(2~{R},3~{S},4~{R},5~{R},6~{S})-2-(hydroxymethyl)-6-[5-(4-methylphenyl)-4~{H}-1,2,4-triazol-3-yl]oxane-3,4,5-triol 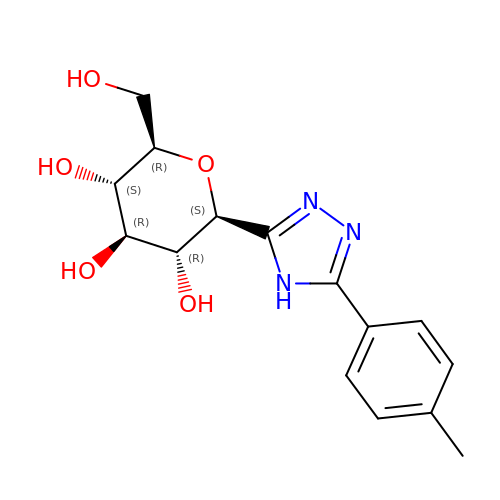| C15 H19 N3 O5 | YAGKTBWCGRXONX-UJPOAAIJSA-N2-[(~{E})-hydroxyiminomethyl]-6-[4-(1,2,3,4-tetrahydroacridin-9-ylamino)butyl]pyridin-3-ol | C23 H26 N4 O2 | 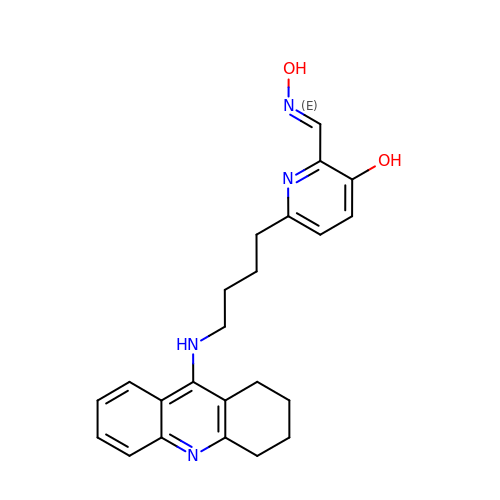WBLSVMZKFSZDDW-MFKUBSTISA-N> MEVKQENRLLNESESSSQGLLGYYFSDLNFQAPMVVTSSTTGDLSIPSSELENIPSENQYFQSAI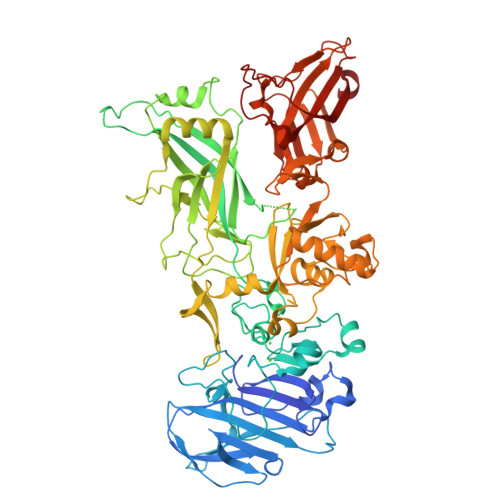WSGFIKVKKSDEYTFATSADNHVTMWVDDQEVINKASNSNKIRLEKGRLYQIKIQYQRENPTEKGLDFKLYWTDSQNKKEVISSDNLQLPELKQKSSNSRKKRSTSAGPTVPDRDNDGIPDSLEVEGYTVDVKNKRTFLSPWISNIHEKKGLTKYKSSPEKWSTASDPYSDFEKVTGRIDKNVSPEARHPLVAAYPIVHVDMENIILSKNEDQSTQNTDSQTRTISKNTSTSRTHTSEVHGNAEVHASFFDIGGSVSAGFSNSNSSTVAIDHSLSLAGERTWAETMGLNTADTARLNANIRYVNTGTAPIYNVLPTTSLVLGKNQTLATIKAKENQLSQILAPNNYYPSKNLAPIALNAQDDFSSTPITMNYNQFLELEKTMQLRLDTDQVYGNIATYNFENGRVRVDTGSNWSEVLPQIQETTARIIFNGKDLNLVERRIAAVNPSDPLETTKPDMTLKEALKIAFGFNEPNGNLQYQGKDITEFDFNFDQQTSQNIKNQLAELNATNIYTVLDKIKLNAKMNILIRDKRFHYDRNNIAVGADESVVKEAHREVINSSTEGLLLNIDKDIRKILSGYIVEIEDTEGLKEVINDRYDMLNISSLRQDGKTFIDFKKYNDKLPLYISNPNYKVNVYAVTKENTIINPSENGDTSTNGIKKILIFSKKGYEIG>MNAAAVTPPPEKFNFAEHLLQTNRVRPDKTAFVDDISSLSFAQLEAQTRQLAAALRAIGVKREERVLLLMLDGTDWPVAFLGAIYAGIVPVAVNTLLTADDYAYMLEHSRAQAVLVSGALHPVLKAALTKSDHEVQRVIVSRPAAPLEPGEVDFAEFVGAHAPLEKPAATQADDPAFWLYSSGSTGRPKGVVHTHANPYWTSELYGRNTLHLREDDVCFSAAKLFFAYGLGNALTFPMTVGATTLLMGERPTPDAVFKRWLGGVGGVKPTVFYGAPTGYAGMLAAPNLPSRDQVALRLASSAGEALPAEIGQRFQRHFGLDIVDGIGSTEMLHIFLSNLPDRVRYGTTGWPVPGYQIELRGDGGGPVADGEPGDLYIHGPSSATMYWGNRAKSRDTFQGGWTKSGDKYVRNDDGSYTYAGRTDDMLKVSGIYVSPFEIEATLVQHPGVLEAAVVGVADEHGLTKPKAYVVPRPGQTLSETELKTFIKDRLAPYKYPRSTVFVAELPKTATGKIQRFKLRE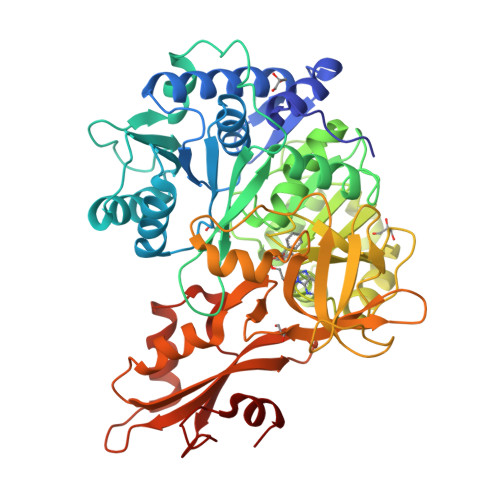GVLG[2x]>[2x]ANPLYQKHIISINDLSRDDLNLVLATAAKLKANPQPELLKHKVIASCFFEASTRTRLSFETSMHRLGASVVGFSDSANTSLG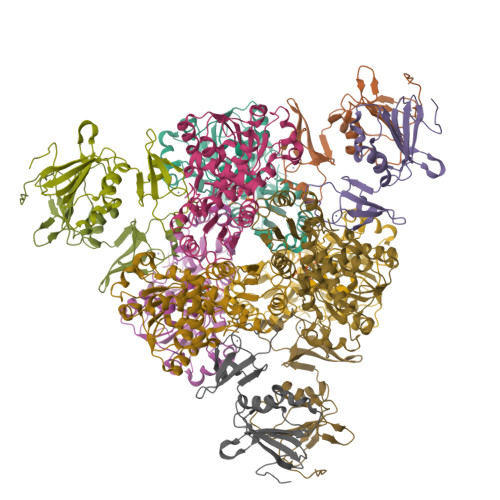KKGETLADTISVISTYVDAIVMRHPQEGAARLATEFSGNVPVLNAGDGSNQHPTQTLLDLFTIQETQGRLDNLHVAMVGDLKYGRTVHSLTQALAKFDGNRFYFIAPDALAMPQYILDMLDEKGIAWSLHSSIEEVMAEVDILYMTRVQKERLDPSEYANVKAQFVLRASDLHNAKANMKVLHPLARVDEIATDVDKTPHAWYFQQAGNGIFARQALLALVLNRDLVL;>MTHDNKLQVEAIKRGTVIDHIPAQIGFKLLSLFKLTETDQRITIGLNLPSGEMGRKDLIKIENTFLSEDQVDQLALYAPQATVNRIDNYEVVGKSRPSLPERIDNVLVCPNSNCISHAEPVSSSFAVRKRANDIALKCKYCEKEFSHNVVLAN[2x]>GMDDETLRLQFGHLIRILPTLLEFEKKGYEPSLAEIVKASG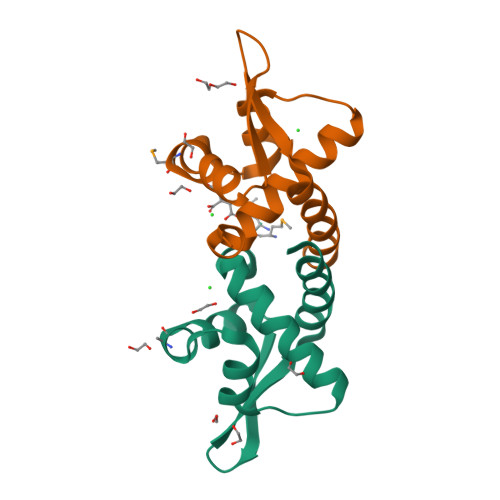VSEKTFFMGLKDRLIRAGLVKEETLSYRVKTLKLTEKGRRLAECLEKCRDVLGS[2x]2-CHLORO-N-(3-CYANO-5,6-DIHYDRO-4H-CYCLOPENTA[B]THIOPHEN-2-YL)-5-DIETHYLSULFAMOYL-BENZAMIDE 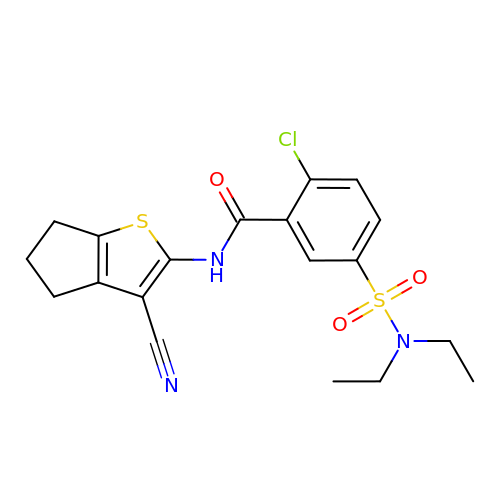| C19 H20 Cl N3 O3 S2 | MZCDQILVXXIMEV-UHFFFAOYSA-N>MLKGKDGVVKNASTGDSIGHLQSWALDTQRDEVSGWGMGDDAERAFTTVGRASGNFEVYLDPADPSDDLEPGDLVDLELYPGGESTGSGYRSVAGALILSTAESASKDGIPMLTVNWRTSGALPQKATVS[6x];>[6x]MQFIDVEFPRDIAAGCQAVLTRRDEVVTLASGREEVNSRWADTRRSWDAGLGVRDEADLAQVVALFEEVRGRLYAFRFRDWLDWRTAATRAPITATDQPLGLGDGSRTAFQVVKVYGAVNPYTRPLSLPHPGTVRVALDGVTQPSGWTLTAPGGVITFDTPPALGVTVTAGCSFDVPVRFSDPELAVQWAYFREGQAGLAQAPSIPLIEVRLDP;>MATVLLAAAGGAIGTSLGGALFGISAAVIGQAVGGLIGQTIDARLSGGGTIKQTGPRLDSLEVMVSQEGTPLADISGRVAVAGTVIWATKLEEIARTTSTRVGSGKSSQKVKSTNFDYAASFAVSLGEGPLNGIGRIFLDGQVRDLSEMISENRVRFYPGTEDQEPDPLIEAIEGAAPAFRGTAYLVFERLFLSDFGNRVPQVRVEVFGQSGEMEKGVTGVCVIPGSTEFGYMPAPVRQQSLDGADVVWEGPENCNRYSRISDWSLSMDHLKNTLPAVQTVSLVVAWFGTDLRAGLCRFEPRIELRAKRTSIEWIAAGLNRGSATEVSRDENDRPAFGSSPADVSVVRAIMDLKARGFRVVLYPFVMMDVTADQALPSPAGTGAQGAYPWRGRIMPDVTGGRVSDQIAALMGTAQPDDFTAAVTRNKSGEISQVNLTCPGAPGDAGLRRFILHLAKLADIAGGVDAFLVGTEFRGLSQAWEPQTYADAYEFLNSSEGWFAQNAARTHEPGSLLVSATARDPRLISPPLSIDGAAARWIEIEFDRTSAPVWEGNVYYMTEDHGFAGAFRKVISDAEAPADGTRARMLLDMHDLTLGGDDWRTSTITRLRFDFSSESDAVFRIHAIRLGGGRRYPFVDALRDLAQDVDTILPTAKISYAADWSEYHSHQDAGDLTFHLDPLWADPAIDFVGIDNYLPLSDWRQGADHLDYDATSGRTTPYDLDYLKSNIEGGEYWDWFYASQEDRDTQTRTPISDGSYGEPWVFRQKAIRDWHANAHHNRTAGVRATTSTGWVPGSKPVWFTEYGCPAVDLGANRPNVFAAASSSESALPWYSSGLRDDFMQRQYLRAMAEWWTANGAPAVDLANCQAWAWDARPFPEFPLRPATWSDGPDWRLGHWLNGRAGAAPAAEAITRRAITRHGLISADIDTSRAYGQADGYAAPAPLGLGDYAQPFEVALGLQTTETGGALVIEAKPAAPLAADVIEADLVDTPAIYTLTRGALEDTPAAAIVRFRDGLSDYEITAARARIGAGKEGGSATADLALVLDGDRGNAAAEMVLRAALTSRESLSVTLPRSATTLRPGSLVEVTLGTEARRLFLVDRVVDGQAREVTLRGFDRAAYAPSGGVFKAARAGRLQGSTSSLTRFLDLPLLPGVDAPEWEGFIAAHAEPWPGAMLHSRGSTPEGSFTLAAEADARATIGRTTAALPPAPAHVWTPGPLVVTLFSGALVGRPDLDVLDGANALAIQHPDGWEVVQFREATLTADRTWRLEGLLRGQRGTDGIVGPAPLPAGAAVVAIDTALVAAGLSADDPGRALWWRSGPDAASLAAAPLRPHTFTAAGLRAFPPAHLRAVVTGGGDTSLSWVPRSRLVGTTWPDNGAPIPSGEGLERYQVTIGPTAAPVRVILADTPAATYTAAERAADGIAAPFRVAVSQISETTGPGPWIETIVTE[3x];>[3x]MTDYTDHLATGCTTLARCYILTRRDGVVMGFTDHDRDIDLDGTRCAAGAALDASTAARSLGITPDDMDAGGALSADAITEADLRAGRYDGAQVEVWEVNWTDPAVRGRLGVYTIGQVERGPLAFRAELRTRPALWNRPEGRIHTALCDVDRLGDHRCKLALGPWQSAATVIEADGADLIVSGLDETASNIFDRGVLDWTGGANAGTGSDIRVARPVAGGVRVSLWSAPPFPITAGDTANATVG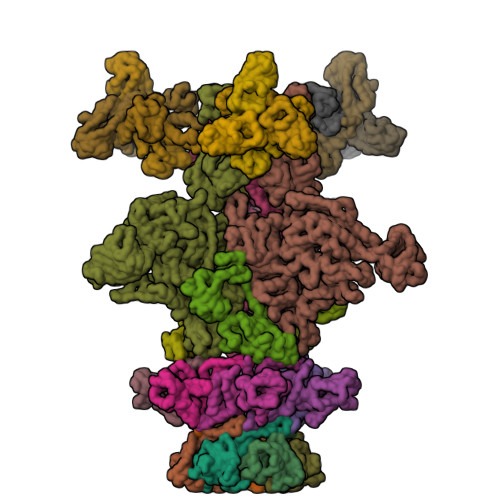CDRTADTCRNRFDNLANFRGFPLMPGESFISEYARPGDPDQSGGSRYD;>[9x]MPTPFLALPLIAEGQAGQHVTHNEALDMIDALAPRVVLSDSLATPPPAPPDRSAWIVPPGGSGFGGAGPGQIALRLGGVWHAITPAQGARWRVLDRGAAVIWSGTSWRPADVSGALGSTLGLATIEATVTATGPSVTAPALIPPRAIVLGVTSWTVQAVTGATSYRVGVPGEPDKFGASLGAAPGSSNIGVVGPFATYAPTDVVVTAEGADFTGGTIGLAASVILPGAPV1-methyl-4-[4-(4-{3-[(piperidin-4-yl)methoxy]pyridin-4-yl}-1H-pyrazol-1-yl)phenyl]piperazine | C25 H32 N6 O | 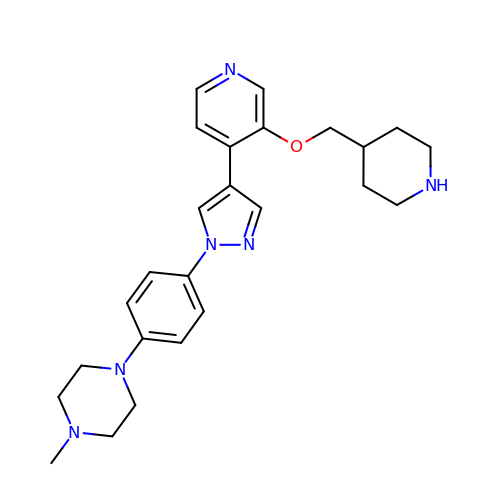BLFBSGVUERKSST-UHFFFAOYSA-N>SMGKLSEQLKHCNGILKELLSKKHAAYAWPFYKPVDASALGLHDYHDIIKHPMDLSTVKRKMENRDYRDAQEFAADVRLMFSNCYKYNPPDHDVVAMARKLQDV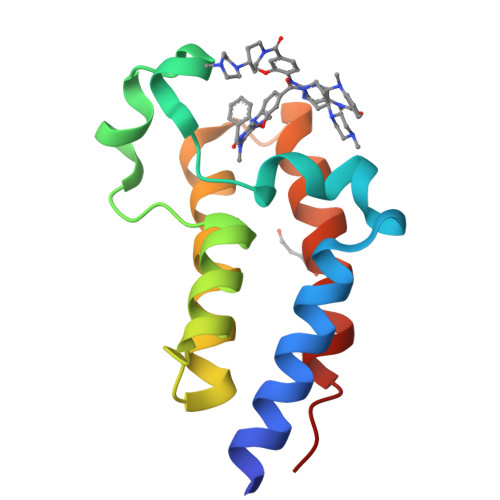FEFRYAKMPD[2x]5'-O-[(R)-[(3,6-dimethyl-2-oxo-1,2-dihydropyridin-4-yl)oxy](hydroxy)phosphoryl]guanosine 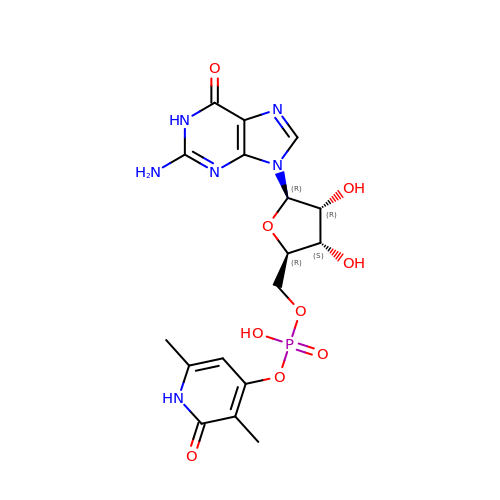| C17 H21 N6 O9 P | SHYVQHDJQQBUQP-UBEDBUPSSA-N>[2x]NAQFLHTQVGRGLLGAVVNPLGEVTDKFAVTDNSEILYRPVDNAPPLYSERAAIEKPFLTGIKVIDSLLTCGEGQRMGIFASAGCGKTFLMNMLIEHSGADIYVIGLIGER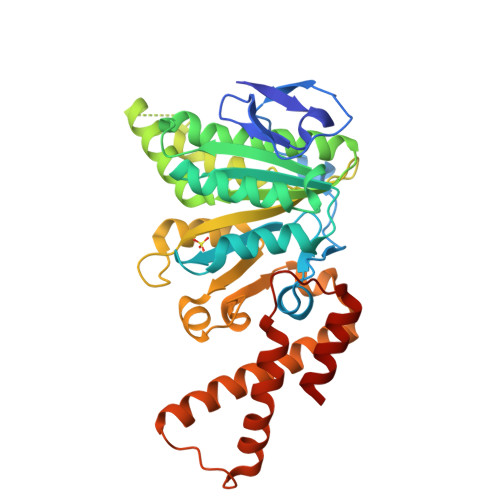GREVTETVDYLKNSEKKSRCVLVYATSDYSSVDRCNAAYIATAIAEFFRTEGHKVALFIDSLTRYARALRDVALAAGESPARRGYPVSVFDSLPRLLERPGKLKAGGSITAFYTVLLEDDDFADPLAEEVRSILDGHIYLSRNLAQKGQFPAIDSLKSISAVFTQVVDEKHRIMAAAFRELLSEIEELRTIIDFGEYKPGENASQDKIYNKISVVESFLKQDYRLGFTYEQTMELIGETIR>GSHGRSRFVKKDGHCNVQFINVGEKRNETLVFSHNAVIAMRDGKLCLMWRVGNLQKSHLVEAHVRAQLLKSRITSEGEYIPLDQIDINVGFDSGIDRIFLVSPITIVHEIDEDSPLYDLSKQDIDNADFEIVVILEGMVEATAMTKQCRSS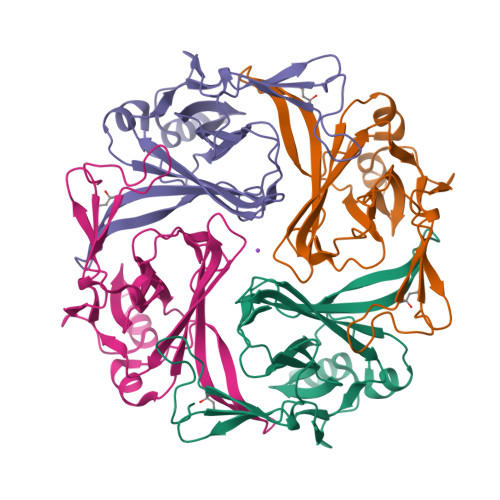YLANEILWGHRYEPVLFEEKHYYKVDYSRFHKTYEVPNTPLCSARDLAEKKYILSNA[4x]(1R)-1-[4-(AMINOCARBONYL)-1,3-THIAZOL-2-YL]-1,4-ANHYDRO-D-RIBITOL | C9 H12 N2 O5 S | 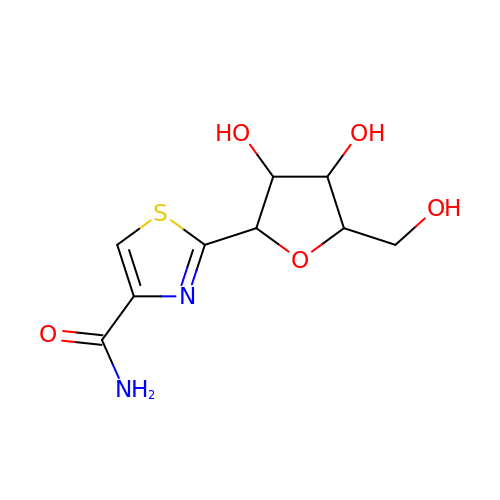FVRDYQYEVDDKCR-DBRKOABJSA-N> MKPIEIHREQPAQHEAMIQLYLDPTLDWFRGHFPVQPLLPGVAQIDWVMHYAQTLLAPGWSFSSIEMVKFQFPLQPGNTLLLKINWDEKKHLLTFRYDLDTHNGSEGQTASQGK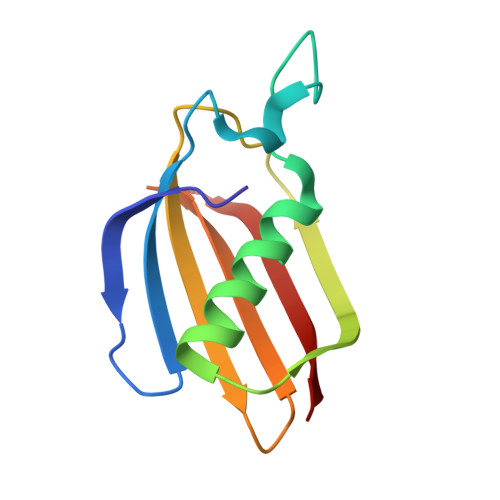IKLCR>[2x]VTQALVKEEIQAKEYLENLNKELAKRTNVETEAAWAYRSAITDENEKKKNEISAELAKFMKEVASDTTKFQWRSYQSEDLKRQFKALTKLGYAALPEDDYAELLDTLSAMESNFAKVKVCDYKDSTKCDLALDPEIEEVISKSRDHEELAYYWREFYDKAGTAVRSQFERYVELNTKAAKLNNFTSGAEAWLDEYEDDTFEQQLEDIFADIRPLYQQIHGYVRFRLRKHYGDAVVSETGPIPMHLLGNMWAQQWSEIADIVSPFPEKPLVDVSAEMEKQAYTPLKMFQMGDDFFTSMN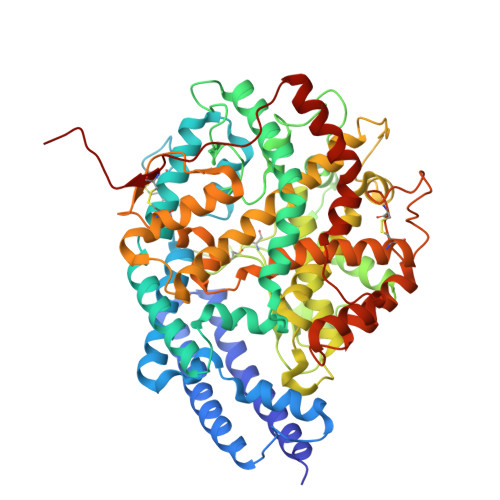LTKLPQDFWDKSIIEKPTDGRDLVCHASAWDFYLIDDVRIKQCTRVTQDQLFTVHHELGHIQYFLQYQHQPFVYRTGANPGFHEAVGDVLSLSVSTPKHLEKIGLLKDYVRDDEARINQLFLTALDKIVFLPFAFTMDKYRWSLFRGEVDKANWNCAFWKLRDEYSGIEPPVVRSEKDFDAPAKYHISADVEYLRYLVSFIIQFQFYKSACIKAGQYDPDNVELPLDNCDIYGSARAGAAFHNMLSMGASKPWPDALEAFNGERIMSGKAIAEYFEPLRVWLEAENIKNNVHIGWITSNKCVSSHHHHH>[2x]MHHHHHHAAGIPMNNPAIKRIGNHITKSPEDKREYRGLELANGIKVLLISDPTTDKSSAALDVHIGSLSDPPNIAGLSHFLQHMLFLGTKKYPKENEYSQFLSEHAGSSNAFTSGEHTNYYFDVSHEHLEGALDRFAQFFLSPLFDESAKDREVNAVDSEHEKNVMNDAWRLFQLEKATGNPKHPFSKFGTGNKYTLETRPNQEGIDVRQELLKFHSAYYSSNLMAVVVLGRESLDDLTNLVVKLFSEVENKNVPLPEFPEHPFQEEHLKQLYKIVPIKDIRNLYVTFPIPDLQKYYKSNPGHYLGHLIGHEGPGSLLSELKSKGWVNTLVGGQKEGARGFMFFIINVDLTEEGLLHVEDIILHMFQYIQKLRAEGPQEWVFQELKDLNAVAFRFKDKERPRGYTSKIAGILHYYPLEEVLTAEYLLEEFRPDLIEMVLDKLRPENVRVAIVSKSFEGKTDRTEEWYGTQYKQEAIPDEVIKKWQNADLNGKFKLPTKNEFIPTNFEILPLEKEATPYPALIKDTAMSKLWFKQDDKFFLPKANLNFEFFSPFAYVDPLHSNMAYLYLELLKDSLNEYAYAAELAGLSYDLQNTIYGMYLSVKGYNDKQPILLK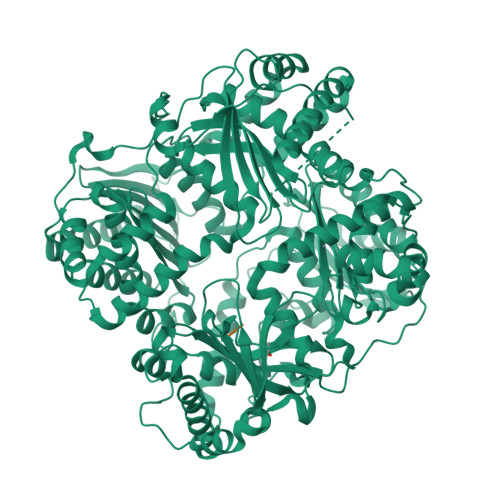KIIEKMATFEIDEKRFEIIKEAYMRSLNNFRAEQPHQHAMYYLRLLMTEVAWTKDELKEALDDVTLPRLKAFIPQLLSRLHIEALLHGNITKQAALGIMQMVEDTLIEHAHTKPLLPSQLVRYREVQLPDRGWFVYQQRNEVHNNSGIEIYYQTDMQSTSENMFLELFAQIISEPAFNTLRTKEQLGYIVFSGPRRANGIQGLRFIIQSEKPPHYLESRVEAFLITMEKSIEDMTEEAFQKHIQALAIRRLDKPKKLSAESAKYWGEIISQQYNFDRDNTEVAYLKTLTKEDIIKFYKEMLAVDAPRRHKVSVHVLAREMDSNPVVGEFPAQNDINLSQAPALPQPEVIQNMTEFKRGLPLFPLVKPHINFMAAKL;>[2x]SPKMVQGSGCFGRKMDRISSSSGLGCKVLRRH> TLIELMIVVAIIGILAAIAIPQY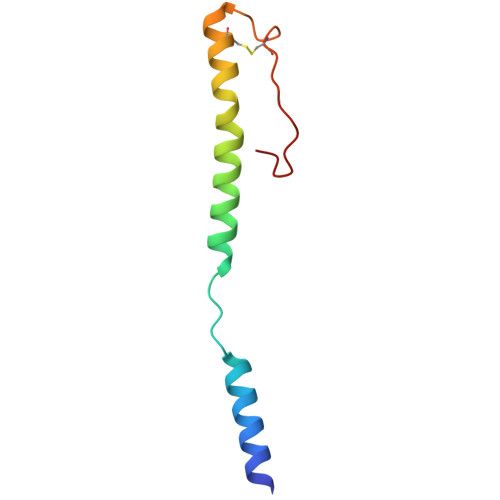QNYIAKSQVSRVMSETGSLKTVIETCILDGKTAANCELGWTNSNLLG> MISNNAPAKMVLNSVLTGYTLAYIQHSIYSDYDVIGRSFWLKEGSNVTRRDFTGIDTFSVTINNLKPTTTYEVQGAFYDSIIDSELLNAQIGINLSDKQTFKMKSAPRITGARCESEPVDVGVGAPIVYIDTTGEADYCTIELKDNSNANNPWVKYYVGALMPTIMFGGVPIGSYKVRISGQISLPDGVTIDSSGYYEYPNVFEVRYNFVPPAAPINIVFKAARIADGKERYDLRVQWDWNRGAGANVREFVLSYIDSAEFVRTGWTKAQKINVGAAQSATIISFPWKVEHKFKVSSIAWGPDAQDVTDSAVQTFILNESTPLDNSFVNETGIEVNYAYIKGKIK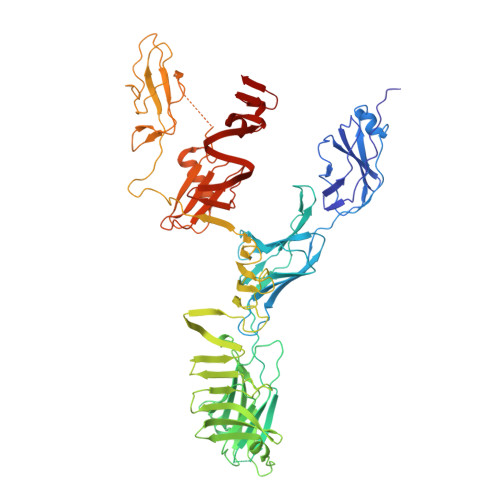DGSTWKQTFLIDAATGAINIGLLDAEGKAPISFDPVKKIVNVDGSVITKTINAANFVMTNLTGQDNPAIYTQGKTWGDTKSGIWMGMDNVTAKPKLDIGNATQYIRYDGNILRISSEVVIGTPNGDIDIQTGIQGKQTVFIYIIGTSLPAKPTSPAYPPSGWSKTPPNRTSNTQNIYCSTGTLDPVTNQLVSGTSWSDVVQWSGTEGVDGRPGATGQRGPGMYSLAIANLTAWNDSQANSFFTSNFGSGPVKYDVLTEYKSGAPGTAFTRQWNGSAWTSPAMVLHGDMIVNGTVTASKIVANNAFLSQIGVNIIYDRAAALSSNPEGSYKMKIDLQNGYIHIR4-chloro-L-tryptophan | C11 H11 Cl N2 O2 | 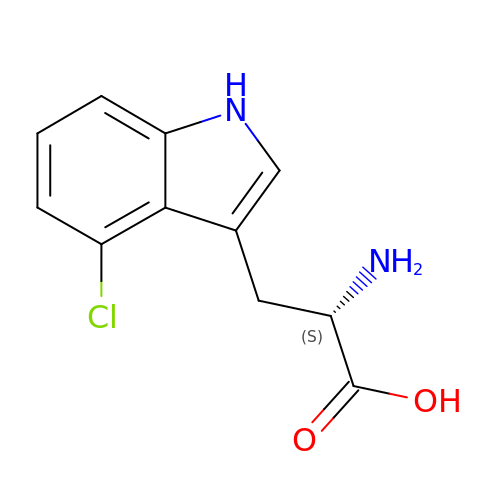NRTHKYABOMUPSC-QMMMGPOBSA-N> VVVQAPTQVPGFLGDSVTLPCYLQVPNMEVTHVSQLTWARHGESGSMAVFHQTQGPSYSESKRLEFVAARLGAELRDASLRMFGLRVEDEGSYTCLFVTFPQGSRSVDIWLRVLAKPQNTAEVQKV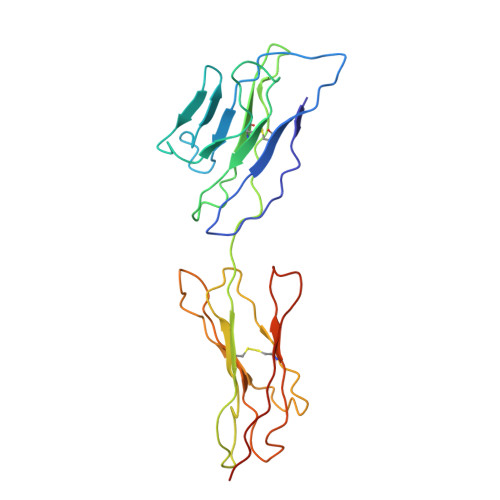QLTGEPVPMARCVSTGGRPPAQITWHSDLGGMPQTSQVPGFLSGTVTVTSLWILVPSSQVDGKQVTCKVEHESFEKPQLLTVSLTVYYPHHHHHH>GSHMHESKEWYHASLTRAQAEHMLMRVPRDGAFLVRKRNEPNSYAISFRAEGKIKHCRVQQEGQTVMLGNSEFDSL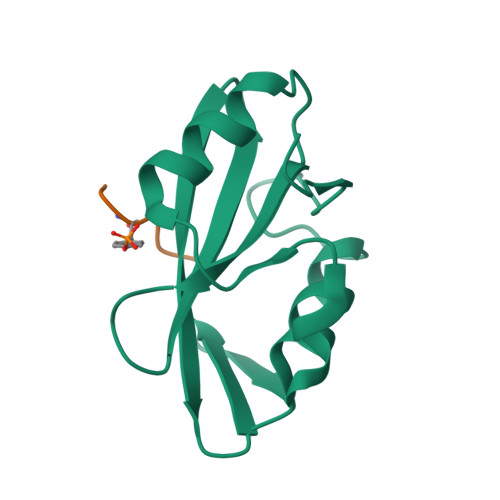VDLISYYEKHPLYRKMKLRYPINEE[4x];>[4x]DNLYYWDQDPP At the core of this natural phenomenon lies a fundamental process of energy transduction by luciferase enzymes that convert the chemical energy stored within the ground-state substrate (luciferin) to an excited, emissive state of the product (oxyluciferin) by a spin-forbidden process. Although beetle luciferase systems share identical substrates and chemical reaction sequence, they emit a range of different colors from yellow green (λmax ≈ 560 nm), which is typical for common firefly species, such as the North American firefly Photinus pyralis (GPp) and the Japanese firefly Luciola cruciata (GLc), to orange and even red (λmax = 590–623 nm) from certain click beetles and railroad worms. Here, we describe the first crystal structures of two rare WT luciferases from Brazilian beetles that emit light with exceptional colors; a luciferase from the head lanterns of the glow-worm P. hirtus (Coleoptera: Phengodidae), the only known luciferase that naturally emits red light (λmax = 623 nm; REPh), and a green-emitting luciferase from the firefly A. vivianii (Coleoptera: Lampyridae) that displays a blue-shifted emission relative to common firefly luciferases (λmax = 538 nm at pH 8; GBAv). Biochemical and structural analyses of the two luciferases, combined with computational modeling, provide the best insight yet into the relationship between the structure and color of light emitted by beetle luciferases.

The crystal structure of WT REPh was determined at low resolution by molecular replacement from two different crystal forms in the space groups P1 and P3121 at resolution of 3.05 Å and 3.60 Å, respectively. Unlike previously reported luciferases that are exclusively monomeric, in the P3121 crystal form, REPh exists as tetramer, although in the P1 crystal form it is an octamer in the asymmetric unit. The N-terminal domains in the octamer core structure are assembled as a tetramer of dimers and packed over dimer and tetramer interfaces, and the C-terminal domains point outward. This assembly accounts for the structural flexibility and increased thermal motion of the C-terminal domains which is apparent from the residual electron density. Only one out of the four C-terminal domains was observed in the density maps of the P3121 crystal form and none of the eight C-terminal domains of the REPh octamer could be resolved in the P1 crystal form. Only molecules C and F of the P1 crystal had sufficient quality in the electron density to trace the complete loop. In the structure of REPh, each dimer within the octamer is stabilized by multiple hydrogen bonds between amino acid residue R11 from one of the monomers and Y26, Y30, and N179 from the other monomers, which extend over a C2 axis across the dimer interface. On the other hand, the hydrophobic interactions between M152, Y153, and F162 from two dimers contribute to the weak overall interactions between the dimers over the tetramer interface.

>[8x]MEEENIVNGDRPRDLVFPGTAGLQLYQSLYKYSYITDGIIDAHTNEVISYAQIFETSCRLAVSLEKYGLDHNNVVAICSENNIHFFGPLIAALYQGIPMATSNDMYTEREMIGHLNISKPCLMFCSKKSLPFILKVQKHLDFLKKVIVIDSMYDINGVECVFSFVSRYTDHAFDPVKFNPKEFDPLERTALIMTSSGTTGLPKGVVISHRSITIRFVHSSDPIYGTRIAPDTSILAIAPFHHAFGLFTALAYFPVGLKIVMVKKFEGEFFLKTIQNYKIASIVVPPPIMVYLAKSPLVDEYNLSSLTEIACGGSPLGRDIADKVAKRLKVHGILQGYGLTETCSALILSPNDRELKKGAIGTPMPYVQVKVIDINTGKALGPREKGEICFKSQMLMKGYHNNPQATRDALDKDGWLHTGDLGYYDEDRFIYVVDRLKELIKYKGYQVAPAELENLLLQHPNISDAGVIGIPDEFAGQLPSACVVLEPGKTMTEKEVQDYIAELVTTTKHLRGGVVFIDSIPKGPTGKLMRNELRAIFAREQAKSKL(1S,2R)-2-[(2S)-2-azanyl-1-oxidanyl-1-oxidanylidene-3-(9H-xanthen-9-yl)propan-2-yl]cyclopropane-1-carboxylic acid | C20 H19 N O5 | 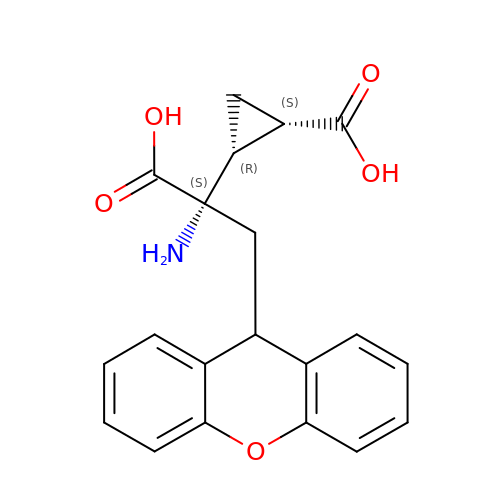VLZBRVJVCCNPRJ-AGKSTNPPSA-N>MVESDSSGIVRHSQGEFDIVQVYKKFLQDDPEITMPVAAIEALVQLLSRSQAKTISEFMDILQNGSNTLKEGVQNNISLSAGCDIFQRFVTRSLHDVGDFEQCKRHLVENGKLFIQRARACRQRIAHLGYPLIRDGSVILTHGFSRGVAAVLLAAAKRHVRFKVFVTESRPSGSGCLMTRTLKNACIPTCMVLDSAVSFTMNRVDLVLVGAEGVVENGGLINQIGTFQLAVFAKHAHKPFYAVAESHKFVRMFPLSQYDIPFSRPILEFDDPSPETVHPEPEPIPTPSDAIHNELIMNEEQIRNNPTLDVTPPEFVSGLITDLGIIDSKSGVSEELIKLYL[2x];>[2x]GPISEFMSTINVEHTYPAVSSLIADLKSRKVQGPFAVAVETALVMRQVISQTRWSTVDQLIDTVRAVGSTLVKAQPTEFSCGNIIRRILRLIREEYQELLKTADENEKLIVSSSNSSSPSQKRDIPSNEKLVQSHEPVSVQMYSSMLNLLGRPTLESPTHSKTVGDSRVTGGMDMRAVIISGIQDVIDELDKINTDIEVQSMDHLHSNEIILTQGCSKTVEAFLRFAAKKRKFSVIVAEGFPNNQKGSHAMAKRLAQAGIDTTVISDATIFAIMSRVNKVILGTHAILGNGGLVTYSGAQLVAQAARHHATPVVVCSGIYKLSPVYPYDLESIIQLSSPDKIMSFNEGDLISRAEILNPYYDYIPPDLVDLFITNLGGYPPSYLYRIMNDTYDASDTIL;>MSLYEHAALPLASSPSILGPISGGRNRGNIQLQSIPIEFQAVVFAGFGNSLYPLTGSDALPKALLPIGNKPMLHYPLYWLEAAGFTSAILICMEEAEAHINAWLRSGYEGHMRIHVEAPTILDDSKSSADALRAVSHLIKNDFVCLSCDSIVGLPPYTVLDKFRLDNPSALAVYSPVLKYEHITSQSKEIDAKQLIGIEEKTSRLLYAKSSADVGSDFTFRMSLLWKHPRVTLNTNLSDAHIFVFKHWVIDLIREKESISSIRGDLIPYLVKCQYQKSFTVRENIQRFLSSPNNIDNYDGGLSSQEIKINALIAKDGIICSRANNLPNYFELNKCIAKLTPEQRLVDVTVSERALVGADCMVNEGTTIKDNSNIKKSIIGKNCVIGKGVVVSNSILMDNIVVEDGVRLESCIVASGAQIGAKSKLRECEIGVDHRVEAGRIARGERLVDMEKIETDMD[2x];>[2x]MGFSAEQAKKDGKDQSPVSESSSVGGTSPATASSVVSPNEPKLSGKEAKALKKARKQASRRAKAEAAAANNPPGVSEEKKVAIPNKNSNQQKKASKQNPQNSPETDANLQEKKIFEEKQVSIFSHLDWRRRRTTENIPKDIHPAVIRLG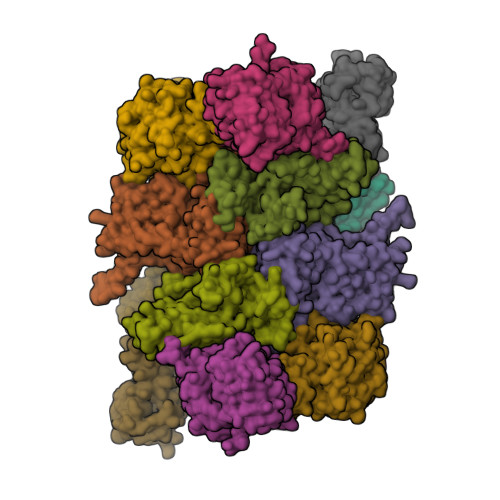LKLANYKIFGSNQRCIDLLKTFKIVIQDYQTPYGTTLSRHLTTHINSQIAYLVSTRPLSISMGNAIRFLKLEISVLDIDLTDDEGKELLLEKIDSYIRDRIIIAGQVIVQAATEKIQDGDVILTYLHSSTVNDVLIHAKNVGKKFRVVVVDSRPEFEGRVCLKLLTEHGIECTYVMISALSYIMQEVTKIFLGGHAMLSNGALYSRAGTSLISLLGHESNVPVIACCESYKFTERIQLDSLVYNELAPGDQLVNMGVDDFEEKPGVLANWKSVKNLKLLSLKYDVTPPRLITVCVCEMGLLPSTSVPAIINEFKQVYA;>MPPSKGLNGKLEKPKHALQAIVLSDSYNYRFRPLTLDKPRCLLPLANTPLIEYTFEFLALAGVQEVYVFCCAHAGQIREYIEKSKWNLPSSPFSVNTIVSRESLSVGDALRELDSKQLITSDFILVSGDVVSNVPLNEVLKEHRKRREDDKNAIMTMVVREASPFHRTRARTESSVFVIDKKTSQCVHYQANERGKHYVSMDPEIFNEHEELEVRNDLIDCQIDICSNDVPALFTENFDYQDIRKDFVYGVLTSDLLGKKIHCHVAKENYAARVRSLQTYDAISKDVLSRWVYPFVPDSNLLNQTFSYQRHQIYKEEDVVLARSCIIKARTLIGAYTKVGDASVVANTIIGRNCTIGSNCSIDSAFLWEDVVIGDNCRIGKAILANSVKIGNNCSIEDGAIVAAGVVIGDNTIIEKNKRLTTFESHSQGTLNDPSLVGIGGRGQEYHAEEDSDDEGEFMEASGLIESTNELHLSDSESSETSSSSEEDMEFIPFSARRDSANTINSEDFDEGDFNKEAQQSLERAFEENHQIDIAALELNTLRMAMNANYHEVRSAIVLALLRRIMHLDVSPKEALAKVMTRWGPLLAKLTFSHEEQVDNVLTLQKYCVRLSMTRHFLQLLGYFYQLEIAEENAIQEWYSDPRSSEGELAALRDAGGKQFVDWLNTAESESESEEGSE[2x];>MSTSHCRFYENKYPEIDDIVMVNVQQIAEMGAYVKLLEYDNIEGMILLSELSRRRIRSIQKLIRVGKNDVAVVLRVDKEKGYIDLSKRRVSSEDIIKCEEKYQKSKTVHSILRYCAEKFQIPLEELYKTIAWPLSRKFGHAYEAFKLSIIDETVWEGIEPPSKDVLDELKNYISKRLTPQAVKIRADVEVSCFSYEGIDAIKDALKSAEDMSTEQMQVKVKLVAAPLYVLTTQALDKQKGIEQLESAIEKITEVITKYGGVCNITMPPKAVTATEDAELQALLESKELDNRSDSEDDEDESDDE[2x]>[2x]TGKCGPPPPIDNGDITSFPLSVYAPASSVEYQCQNLYQLEGNKRITCRNGQWSEPPKCLHPCVISREIMENYNIALRWTAKQK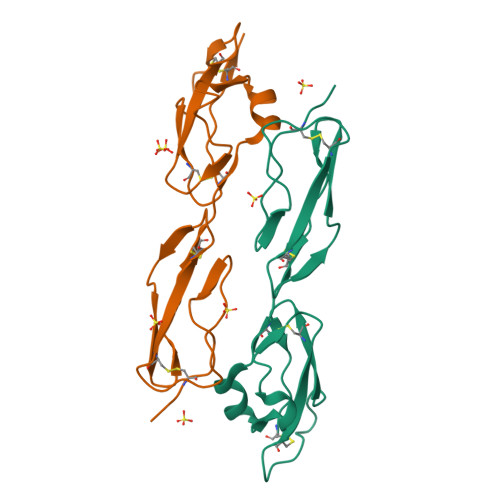LYLRTGESAEFVCKRGYRLSSRSHTLRTTCWDGKLEYPTCAK> SNAQDENYTTPIVSSAALTKENQCEWGQWESFKQHYIENGRVVDNSDPRLITTSEGQSYALFFA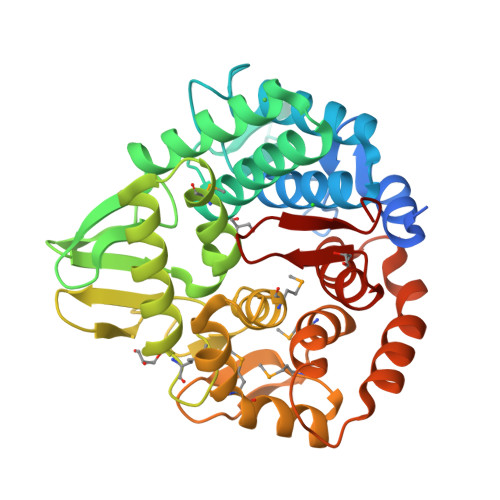LIANDKKTFDELLGWTELHLAGGDLTAQLPAWLWGTQPDGSQGILDSNSAADSDLWIAYSLLEAGRLWDNHYYQSLGHLLASRILRDETIKVSGLGTVLLPGKVGFVLGKNHVRLNPSYVPLQLLTRMNTVFPSYQWEEIYQSSAKLLKETMPKGYSPDWVEWDKTQFKKDSKAQSVGSYNAIRVYLWAGMLPDSDPNKALLLGKMKPLLRVIERNKGMPETINVLTGKGKNQGGVGMNAAILPLLSSLDSNTNVAEYEKKIQAELPKIESDYYYNSVLTLFGLGWYQDLYSFNDDGSVTPKWVNVCQ>MSRRNPCKFEIRGHCLNGKRCHFSHNYFEWPPHALLVRQNFMLNRILKSMDKSIDTLSEISGAAELDRTEEYALGVVGVLESYIGSINNITKQSACVAMSKLLTELNSDDIKKLRDNEELNSPKIRVYNTVISYIESNRKNNKQTIHLLKRLPADVLKKTIKNTLDIHKSITINNPKESTVSDTNDHAKNNDTT[4x];>[4x]DPTPSDNPFSKLYKET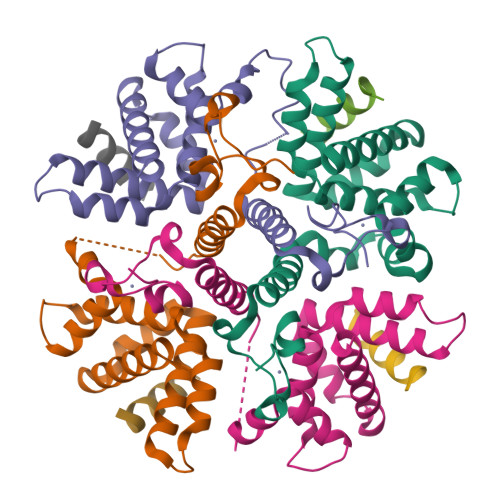IETFD>LIQERRSHEVNPAAHLTGANSS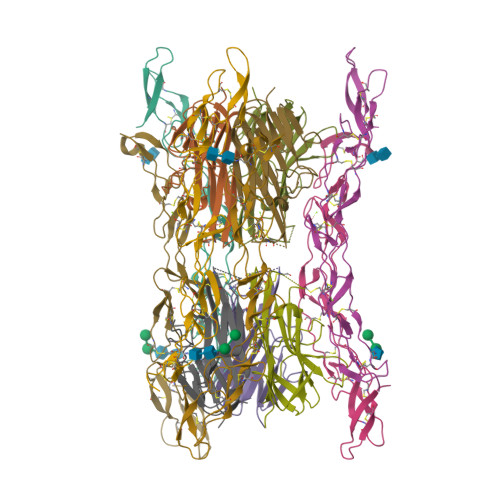LTGSGGPLLWETQLGLAFLRGLSYHDGALVVTKAGYYYIYSKVQLGGVGCPLGLASTITHGLYKRTPRYPEELELLVSQQSPCGRATSSSSNWFDSSFLGGVVHLEAGEEVVVRVLDERLVRLRDGTRSYFGAFMV[2x];>[2x]VAETPTYPWRDAETGERLVCAQCPPGTFVQRPCRRDSPTTCGPCPPRHYTQFWNYLERCRYCNVLCGEREEEARACHATHNRACRCRTGFFAHAGFCLEHASCPPGAGVIAPGTPSQNTQCQPCPPGTFSASSSSSEQCQPHRNCTALGLALNVPGSSSHDTLCTSTGHHHHHH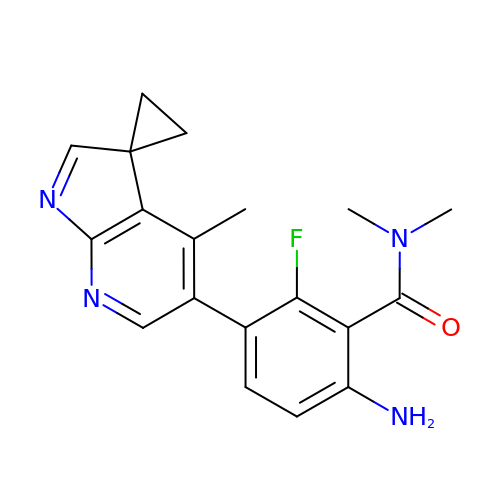6-amino-2-fluoro-N,N-dimethyl-3-(4'-methylspiro[cyclopropane-1,3'-pyrrolo[2,3-b]pyridin]-5'-yl)benzamide | C19 H19 F N4 O | MPBBKYMTAPEIGF-UHFFFAOYSA-N> MIERLNSPFLRAAALFTIVAFSSLISTAALAENNPSDTAKKFKVVTTFTIIQDIAQNIAGDVAVVESITKPGAEIHDYQPTPRDIVKAQSADLILWNGMNLERWFEKFFESIKDVPSAVVTAGITPLPIREGPYSGIANPHAWMSPSNALIYIENIRKALVEHDPAHAETYNRNAQAYAEKIKALDAPLRERLSRIPAEQRWLVTSEGAFSYLAKDYGFKEVYLWPINAEQQGIPQQVRHVIDIIRENKIPVVFSESTISDKPAKQVSKETGAQYGGVLYVDSLSGEKGPVPTYISLINMTVDTIAKGFGQLEHHHHHHHHHH

YfeA is a polyspecific cluster A-1 SBP that is important for Y. pestis infection and transition-metal homeostasis. Biochemical analysis indicates that the Yfe system transports manganese and iron, and complements their respective transporters MntH and FeoABC. At the arch of the c-clamp is a tetracoordinate canonical site composed of His76, His141, Glu207 and Asp282.

By varying the protein-expression conditions, we observed crystallization of YfeA in three crystal forms. In this report, the lattices with edges 42 × 52 × 113, 62 × 66 × 67 and 55 × 67 × 82 Å will be referred to as crystal forms 1, 2 and 3, respectively. The structure of crystal form 1 was solved by single anomalous dispersion (SAD), and the structures in the other crystal forms were determined by molecular replacement (MR). free of 17.88 and 19.03%, respectively, and used for MR and refinement of crystal form 2 and crystal form 3. The high-quality diffraction data enabled the resolution of holes in aromatic and proline residues. Although this observation suggests that the primary ligand at site 1 is zinc, further inspection was needed as nutrient-rich conditions contain unequal abundances of free metals in solution, and zinc is the most abundant transition metal in LB. The inter­atomic distances of site 1 ligands are 3.0 Å ≤ x–x1 ≤ 3.6 Å. Based on this analysis, the interatomic distances of site 1 ligands can integrate zinc, iron and manganese, further supporting the hypothesis that YfeA site 1 is polyspecific.>[4x]GSHMADSSSSSFFPDFGLLLYLEELNKEELNTFKLFLKETMEPEHGLTPWNEVKKARR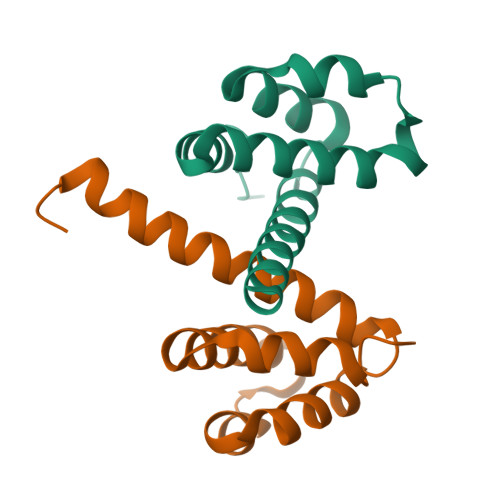EDLANLMKKYYPGEKAWSVSLKIFGKMNLKVLCERAKEEINWSAQLE> MNGIHDTGGAHGYGPVYREPNEPVFRYDWEKTVMSLLPALL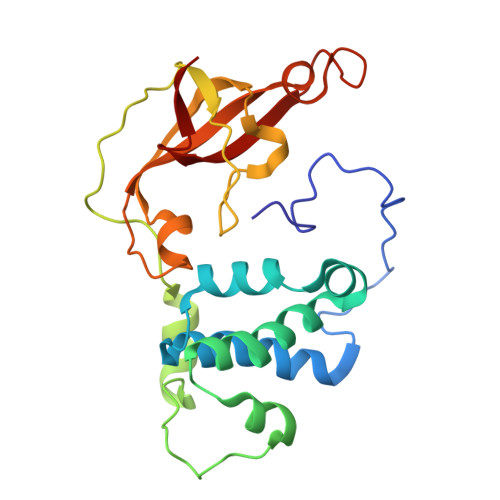ANGNFNLDEFRHSIERMGPAHYLEGTYYELWLHVFENLLVEKGVLTATEVATGKAASGKTATPVLTPAIVDGLLSTGASAAREEGARARFAVGDKVRVLNKNPVGHTRMPRYTRGKVGTVVIDHGVFVTPDTAAHGKGEHPQHVYTVSFTSVELWGQDASSPKDTIRVDLWDDYLEPA> MGMATYAVVDLETTGNQLDFDDIIQIGITFVRNNQIIDTYHSMIRTNLEIPPFIQALTSIEENMLQQAPYFNQVAQEIYDKIKDCIFVAHNVDFDLNFIKKAFKDCNIQYRPKKVIDTLEIFKIAFPTDKSYQLSELAEAHGITLANAHRADEDAATTAKLMILAFEKFEKLPLDTLKQLYYLSKQLKYDLYDIFFEMVRQYDAKPLDKFYEKFEQIIYRKQVDFKKPTTNYNGSLKSLYRKAVDQLGLTYRPQQLYLAETILDQLMHSEKAMIEASLGSGKSLAYLLAALMYNIETGKHVMISTNTKLLQSQLLEKDIPAMNEALNFKINALLIKSKSDYISLGLISQILKDDTSNYEVNILKMQLLIWITETPSGDIQELNLKGGQKMYFDQKIETYVPARHDVHYYNFIKRNAQNIQIGITNHAHLIHSDVENSIYQLFDDCIVDEAHRLPDYALNQVTNELSYADIKYQLGLIGKNENEKLLKAIDQLEKQRILEKLDIAPIDIFGLKASMNEIHELNEQLFSTIFTIINDSDVYDDDIHRFHNVFTFETKDILKDLHAIIDKLNKTLEIFNGISHKTVKSLRKQLLYLKDKFKNIEQSLKAGHTSFISIKNLSQKSTIRLYVKDYAVKDVLTKQVLEKFKSLIFISGTLKFNHSFEAFKQLFNKDVHFNTFEVNTSLQSAKNTSVFIPSDVASYQYKNIDEYVASIVSYIIEYTTITSSKCLVLFTSYKMMHMVQDMLNELPEFEDYVVLTQQQNQNYKIVQQFNNFDKAILLGTST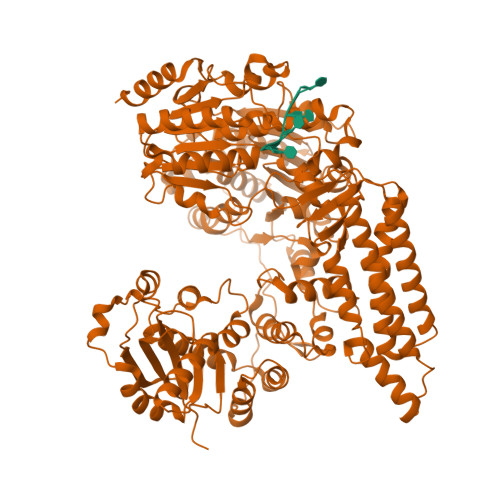FFEGFDFQANGIKCVMIAKLPFMNKHNAKYWLMDSEFTSTFKEYVLPDAVTRFRQGLGRLIRNENDRGIIVSFDDRLINSNYKNFFEQTLENYRQKKGDIQQFGKLLRQIQKKKK ANTIMYCIN | C27 H38 N2 O9 | 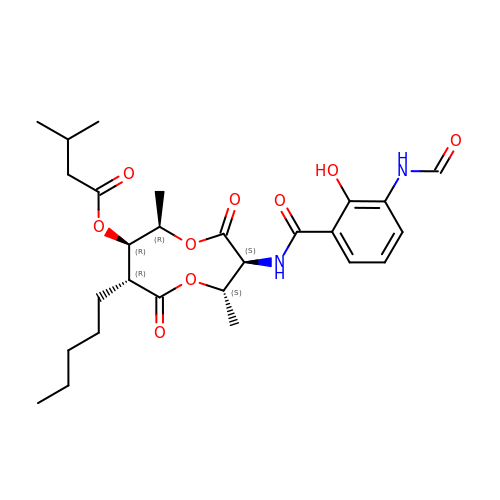ZVYMCLIDNNTNCL-BJDKEMKCSA-N> GADLADRFAELERRYDARLGVYVPATGTTAAIEYRADERFAFCSTFKAPLVAAVLHQNPLTHLDKLITYTSDDIRSISPVAQQHVQTGMTIGQLCDAAIRYSDGTAANLLLADLGGPGGGTAAFTGYLRSLGDTVSRLDAEEPELNRDPPGDERDTTTPHAIALVLQQLVLGNALPPDKRALLTDWMARNTTGAKRIRAGFPADWKVIDKTGTGDYGRANDIAVVWSPTGVPYVVAVMSDRAGGGYDAEPREALLAEAATCVAGVLA

BlaC is a broad-spectrum β-lactamase which confers resistance to all classes of β-lactam antibiotics in tuberculosis. BlaC from M. tuberculosis, an Ambler class A β-lactamase, uses a conserved serine to attack the β-lactam ring (blue arrow), thus inactivating the antibiotics. Specifically, we have obtained time-resolved crystallographic data on the binding and cleavage of the third-generation antibiotic ceftriaxone (CEF) in microcrystals of the enzyme β-lactamase from Mycobacterium tuberculosis (BlaC). In our MISC experiment, the small microcrystals were rapidly mixed with CEF “on the fly” using optimized mixing devices, and structures of the reaction of BlaC with CEF were determined by scattering from femtosecond X-ray pulses at five time points (unmixed, and 30 ms, 100 ms, 500 ms, and 2 s after mixing, respectively) during the reaction in both crystal forms.

We have therefore crystallized BlaC in two different crystal forms. With polyethylene glycol (PEG) 1000 as the precipitant, needle-shaped crystals are obtained with one molecule in the asymmetric unit. The solvent volume as estimated by the CCP4 program “truncate” is on the order of 59% for the shard-shaped crystal, and it is substantially lower (28%) in the needles. When measured by the program Coot, cavities with diameters as wide as 90 Å can be identified in the shards, and only 20-Å voids exist in the needles. The reason for this might be that the enzyme is more tightly packed in the needle crystal form. Since stacking is not observed in crystals that pack in the same way as our needle crystal form, it might be argued that it represents a non-physiological, non-specifically bound substrate that occurs only in the environment in the shard crystals.>[2x]VPLLRHDPLLRLTLELLRPR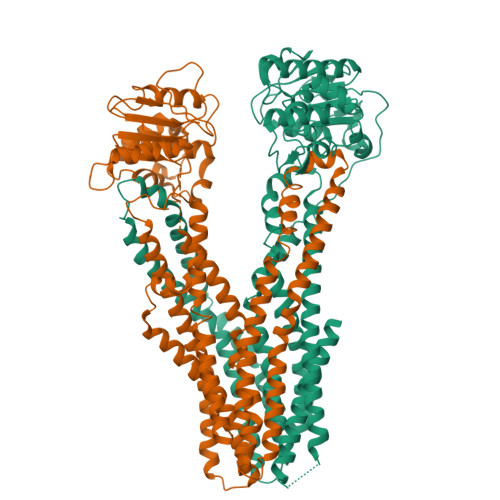LGRFLLAAALGVLSLGSALALAGISAWLITRAWQMPPVLDLTVAVVAVRALGISRGVLGYCQRLASHDSALRAAANARTGLYRKLADAPPDEAMRLPSGELVARLGPAVDELADVLVRALLPIVVAVVLGCAAVGVIAVISPASAAVLAVCLVVAGVVAPALAARAAHASETVAAEHRSQRDTAGMLALEHAPELRVSGRLDSVIATFERHHRAWGEAADRAAAPAAVAAAMPTAAMGVSVVGAVIAGIALAPTVAPTTAAILMLLPLSAFEATTALPDAAAQLMRSRVAARRLLELTTPTPLRSRPDVATVDLAPGDRLAVVGPSGSGKTTMLMAIADRLNGAGGETPQRAAVFAEDAHLFDTTVRDNLLVVRGDATDTELVAALDRVGLGEWLAGLPDGLSTVLVGGAAAVSAGQRRRLLIARALISAFPVVLLDEPTENLDAGDARQMLEGLLTPGALFAADRTVVVATHHLPPGFDCPIVRCTGRLAVAGRYLGGIKAFDYKDDDDK;>[2x]SYFQSNVVIAGCTIASAVVLAHIVAGIITNPATALGGETDWAPGLVALAVLWSVRVVAQWFQGRLSQRGATAVIGELSRQVLSSVTTSSPRRLAADRDSAAAVVTRGLDGLRPYFTGYLPAVVLAGILTPAALVVMAAYDWQAAAIVVIALPLIPIFMVLIGLLTAERSAAALTAMTTLQGRMLDLIAGIPTLRAVGRAGGSVQRIAELSASHRRSTMATLRISFLSALVLELLATLGVALVAVSVGLRLVFGDMTLAAGLTALLLAPEVFWPLRRVGAAFHAAQDGKTAAEQALRLCAEPHPPTGHEVVPAGAPVIEVPALKAVMEPGRVTVLTGPNGVGKSTLLQAILGLQESPCGPILVAGVEVGALDRSAWWGRLAWMPHRPVLVPGTVRENLELLGPVPGLDEVCRSVGFDEVLGELPDGSETPLGRGGVGLSLGQRQRLGLVRALGAPADVLLLDEPTAHLDGALEDRVLAAIVARARAGATVVMVGHRAPVLAAADHVVTMESSLVAP> GP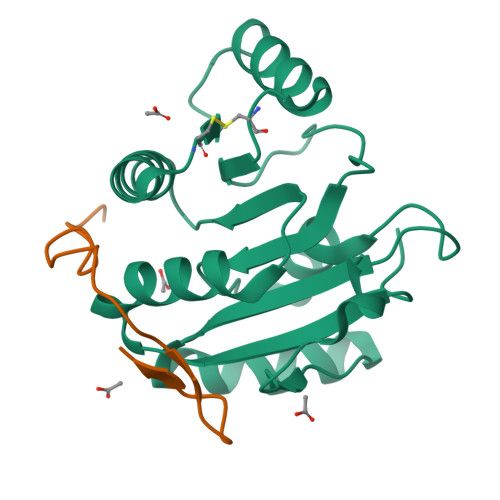HMELTLKGVTQYYAFVQERQKVHCLNTLFSKLQINQSIIFCNSTQRVELLAKKITELGYCCYYIHAKMAQAHRNRVFHDFRQGLCRNLVCSDLFTRGIDVQAVNVVINFDFPRMAETYLHRIGRSGRFGHLGIAINLITYEDRFDLHRIEKELGTEIKPIPKVIDPALYV;> DENLPEWAIENPSKLGGSFDASGAFHG N-[2-(2-chlorophenyl)-4-methyl-5-(1-methylethyl)-1H-imidazol-1-yl]-5-methyl-2,3-dihydro-1,4-benzodioxine-6-carboxamide 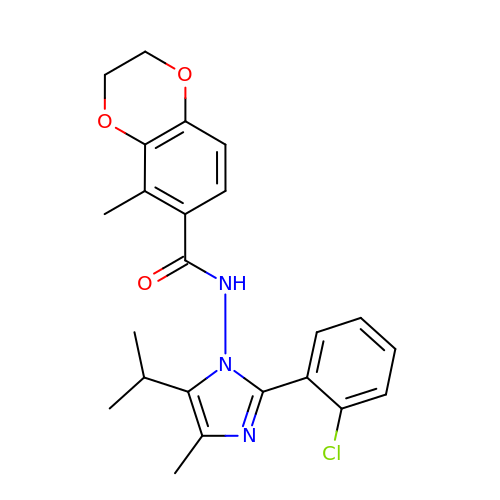| C23 H24 Cl N3 O3 | XLNQTHXOKGRTAL-UHFFFAOYSA-N>[3x]GPGSMVSELNGDTEPEVLVEQRDRILIITINRPKAKNSVNAAVSRALADAMDRLDADAGLSVGILTGAGGSFCAGMDLKAFARGENVVVEGRGLGFTERPPAKPLIAAVEGYALAGGTELALATDLIVAARDSAFGIPEVKRGLVAGGGGLLRLPERIPYAIAMELALTGDNLSAERAHALGMVNVLAEPGAALDAAIALAEKITANGPLAVAATKRIITESRGWSLDT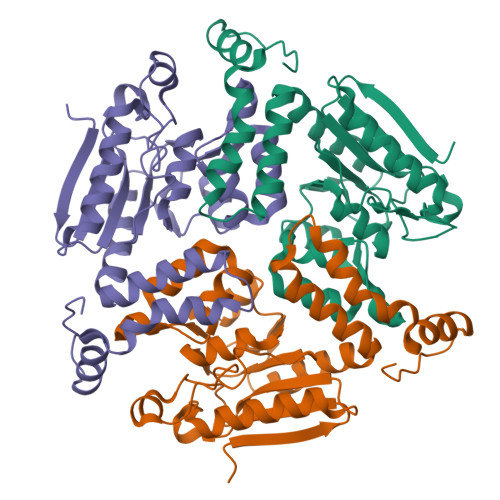RFAQQMKILFPIFTSNDAKEGAIAFAEKRPPRWTGT>UUGGGCCUGCUGCUGGUCC[2x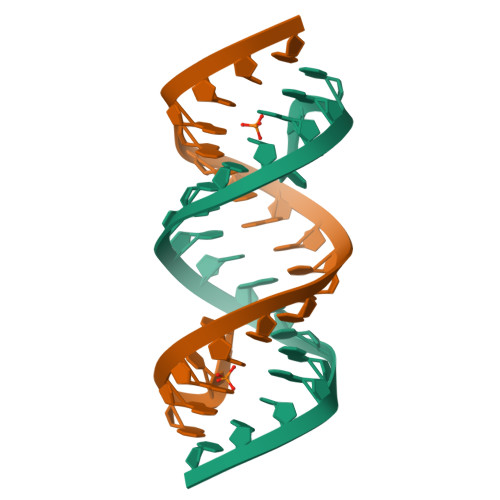]> SNAVDLSDADTLQRYLDQRFQQVDVSVKLELWHEAYRSIEDVFHLMKISKRAPKPSTLANYYENLVKVFFVSGDPLLHTTAWKKFYKLYSTNPRATEEEFKTYSSTIFLSAISTQLDEIPSIGYDPHLRMYRLLNLDAKPTRKEMLQSIIEDESIYGKVDEELKELYDIIEVNFDVDTVKQQLENLLVKLSSKTYFSQYIAPLRDVIMRRVFVAASQKFTTVSQSELYKLATLPAPLDLSAWDIEK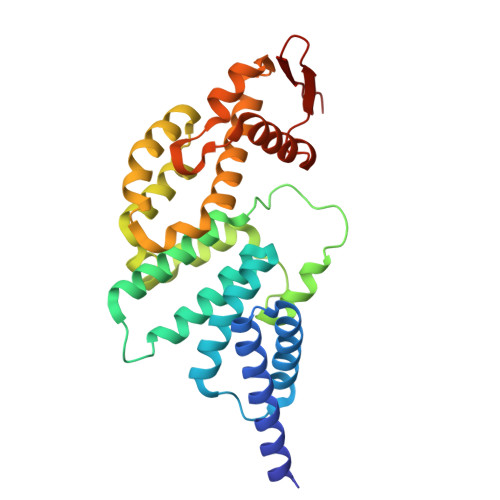SLLQAAVEDYVSITIDHESAKVTFAKDP>[2x]MGGSSHHHHHHS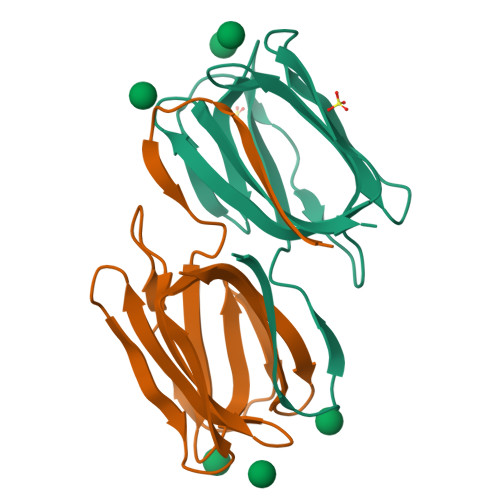SGLVPRGSGGLTHRKFGGSGGSPFSGLSSIAVRSGSALDAIIIDGVHHGGSGGNLSPTFTFGSGEYISNMTIRSGDAIDNISFETNMGRRFGPYGGSGGSANTLSNVKVIQINGSAGDALDSLDIYYEQY>[2x]LPSGSDPAFSQPKSVLDAGLTCQGASPSSVSKPILLVPGTGTTGPQSFDSNWIPLSTQLGYTPCWISPPPFMLNDTQVNTEYMVNAITALYAGSGNNKLPVLTWSQGGLVAQWGLTFFP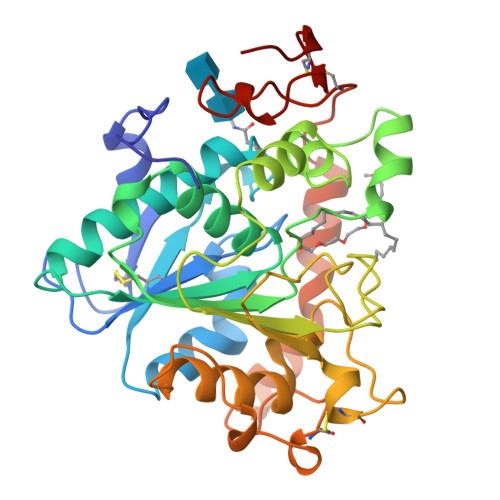SIRSKVDRLMAFAPDYKGTVLAGPLDALAVSAPSVWQQTTGSALTTALRNAGGLTQIVPTTNLYSATDEIVQPQVSNSPLDSSYLFNGKNVQAQAVCGPLFVIDHAGSLTSQFSYVVGRSALRSTTGQARSADYGITDCNPLPANDLTPEQKVAAAALLAPAAAAIVAGPKQNCEPDLMPYARPFAVGKRTCSGIVTP>MAKGDVITLNFETFVDSDTQVKVTRLTPTDIICHRNYFYQKCFTQDGKKLLFAGDFDGNRNYYLLNLETQQAVQLTEGKGDNTFGGFISTDERAFFYVKNELNLMKVDLETLEEQVIYTVDEEWKGYGTWVANSDCTKLVGIEILKRDWQPLTSWEKFAEFYHTNPTCRLIKVDIETGELEVIHQDTAWLGHPIYRPFDDSTVGFCHEGPHDLVDARMWLVNEDGSNVRKIKEHAEGESCTHEFWIPDGSAMAYVSYFKGQTDRVIYKANPETLENEEVMVMPPCSHLMSNFDGSLMVGDGCDAPV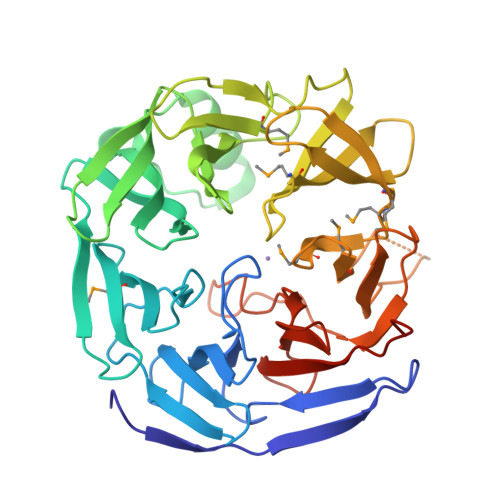DVADADSYNIENDPFLYVLNTKAKSAQKLCKHSTSWDVLDGDRQITHPHPSFTPNDDGVLFTSDFEGVPAIYIADVPESYKHLEHHHHHH[3x]>[3x]ADDEDCCSYEDRREIRHIWDDVWSSSFTDRRVAIVRAVFDDLFKHYPTSKALFERVKIDEPESGEFKSHLVRVANGLKLLINLLDDTLVLQSHLGHLADQHIQRKGVTKEYFRGIGEAFARVLPQVLSCFNVDAWNRCFHRLVARIAKDLP;>KKQCGVLEGLKVKSEWGRAYGSGHDREAFSQAIWRATFAQVPESRSLFKRVHGDDTSHPAFIAHADRVLGGLDIAISTLDQPATLKEELDHLQVQHEGRKIPDNYFDAFKTAILHVVAAQLGRCYDREAWDACIDHIEDGIKGHH[3x];>[3x]DEHEHCCSEEDHRIVQKQWDILWRDTESSKIKIGFGRLLLTKLAKDIPEVNDLFKRVDIEHAEGPKFSAHALRILNGLDLAINLLDDPPALDAALDHLAHQHEVREGVQKAHFKKFGEILATGLPQVLDDYDALAWKSCLKGILTKISSRLNA;>ECLVTESLKVKLQWASAFGHAHERVAFGLELWRDIIDDHPEIKAPFSRVRGDNIYSPEFGAHSQRVLSGLDITISMLDTPDMLAAQLAHLKVQHVERNLKPEFFDIFLKHLLHVLGDRLGTHFDFGAWHDCVDQIIDGIK[3x];> RFQYLVKNQNLHIDYLAKKLHDIEEEYNKLTHDVDKKTIRQLKARISNLEEHHCDEHESECRGDVPECIHDLLFCDGEKDCRDGSDEDPETCSLNITHV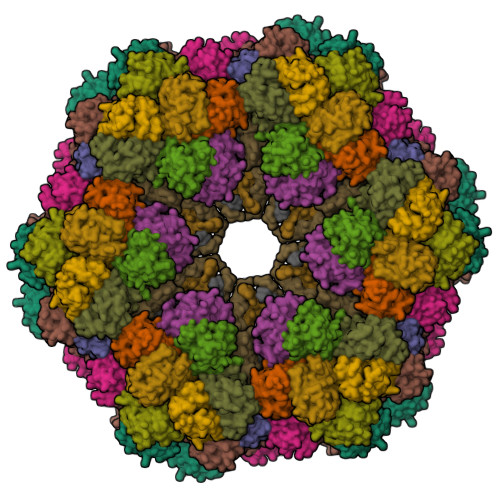GSSYTGLATWTSCEDLNPDHAIVTITAAHRKSFFPNRVWLRATLSYELDEHDHTVSTTQLRGFYNFGKRELLLAPLKGQSEGYGVICDFNLGDDDHADCKIVVPSSLFVCAHFNAQRY;> LDPRLGANAFLIIRLDRIIEKLRTKLDEAEKIDPEHFVSEIDARVTKIEGTHCEKRTFQCGGNEQECISDLLVCDGHKDCHNAHDEDPDVCDTSVVKAGNVFSGTSTWHGCLAREDHVTRITITASKRRKFFTARIWLRALVESELERHGENVTSSFNAKGYYNFASRRLILLPTDDHDDHLAVVCSFNRGDNERAECHRVTEATLHQCADLFVTLEEHD;> QSHDEIIDKLIERTNKITTSISHVESLLDDRLDPKRIRKAGSLRHRVEELEDPSCDEHEHQCGGDDPQCISKLFVCDGHNDCRNGEDEKDCTLPTKAGDKFIGDVCFDHCTKRRPEHMTLAFESSSIAAFFTPIADLHVHIEIESETDEDESEVSMPADGEYSFADHRLTIHPPEEDGLGLVGEFDGYNFDRFVGHIVHELSEEVCAEFIFHRKK>MRGSHHHHHHGSAVHHPPSYVARLASDFGVRVFQQVAQASKDRNVVFSPYGVASVLAMLQLTTGGETQQQIQAAMGFKIDDKGMAPALRHLYKELMGPWNKDEISTTDAIFVQRDLKLVQGFMPHFFRLFRSTVKQVDFSEVERARFIINDWVKTHTKGMISHLLGTGAVDQLTRLVLVNALYFNGQWKTPFPDSSTHRRLFHKSDGSTVSVPMMAQTNKFNYTEFTTPDGHYYDILELPYHGDTLSMFIAAPYEKEVPLSALTNILSAQLISHWKGNMTRLPRLLVLPKFSLETEVDLRKPLE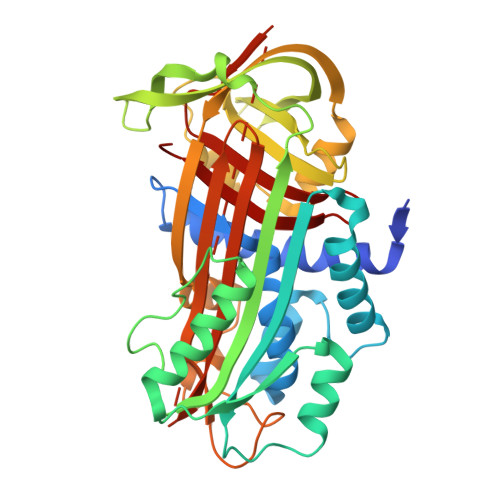NLGMTDMFRQFQADFTSLSDQEPLHVALALQKVKIEVNESGTVASSSTAVIVSARMAPEEIIIDRPFLFVVRHNPTGTVLFMGQVMEP[2x]>MLVFIDDGSTNIKLQWQESDGTIKQHISPNSFKREWAVSFGDKKVFNYTLNGEQYSFDPISPDAVVTTNIAWQYSDVNVVAVHHALLTSGLPVSEVDIVCTLPLTEYYDRNNQPNTENIERKKANFRKKITLNGGDTFTIKDVKVMPESIPAGYEVLQELDELDSLLIIDLGGTTLDISQVMGKLSGISKIYGDSSLGVSLVTSAVKDALSLARTKGSSYLADDIIIHRKDNNYLKQRINDENKISIVTEAMNEALRKLEQRVLNTLNEFSGYTH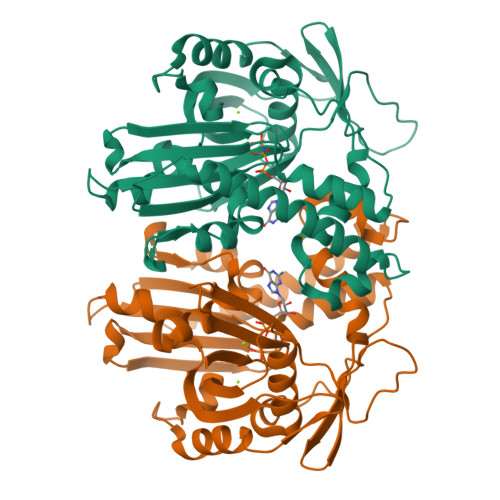VMVIGGGAELICDAVKKHTQIRDERFFKTNNSQYDLVNGMYLIGN[2x]Here, by deleting the branch-site adenosine (BS-A) or mutating the branch-site sequence of an actin pre-mRNA, we stall the assembly of spliceosomes in extracts from the yeast Saccharomyces cerevisiae directly before the A complex is formed. We then determine the three-dimensional structure of this newly identified assembly intermediate by cryo-electron microscopy. Our structure indicates that the U2–BS helix has formed in this pre-A complex, but is not yet clamped by the HEAT domain of the Hsh155 protein (Hsh155HEAT), which exhibits an open conformation. Thus, Prp5 proofreads the branch site indirectly, hindering spliceosome assembly if branch-site mutations prevent the remodelling of Hsh155HEAT.

To isolate a spliceosome assembly intermediate formed directly before the A complex that still contains Prp5, we carried out splicing in S. cerevisiae cell extracts with an actin (Act) pre-mRNA in which the BS-A is deleted. Spliceosomal complexes formed on ΔBS-A Act pre-mRNA lack the U4/U6.U5 tri-snRNP, but contain stoichiometric amounts of U1 and U2 snRNPs. The proteins Prp5, Msl5 and Mud2 are also abundant, whereas Cus2 is absent, indicating that these complexes stall after Prp5 hydrolyses ATP, but before the tri-snRNP has docked. We next carried out single-particle cryo-electron microscopy (cryo-EM) and determined the structure of the ΔBS-A complex at an average resolution of 5.9 Å (ranging from roughly 4.5 Å for U1 to approximately 15 Å for U2). By fitting known X-ray structures of spliceosome components into the EM density map, together with protein crosslinking coupled with mass spectrometry (CXMS), we generated a three-dimensional (3D) model of the ΔBS-A complex. This complex consists of two major elongated domains—comprising the U1 and bipartite U2 snRNPs—that are connected by two main bridges. In the pre-A complex, U1 and U2 are connected by a second bridge comprising intron nucleotides upstream of the branch site. Thus, formation of the U2–BS helix alone does not appear to trigger closure of Hsh155HEAT. As the U2–BS helix has formed, but Hsh155HEAT still exhibits an open conformation and Prp5 is stably bound (see below), we conclude that ΔBS-A complexes are stalled at a pre-A-complex stage, after Prp5-mediated formation of the U2–BS helix, but during/before it carries out its proofreading function. Comparison of our pre-A complex with the previously published yeast A complex15 reveals that the transition from the pre-A to the A complex involves large-scale remodelling that requires displacement of Prp5. The repositioning of U1 and the U2 3′-region is essential to generate the binding platform needed to dock the U4/U6.U5 tri-snRNP during formation of the pre-B complex.

> MSALYFQNLPSRPANKENYTRLLLKHINPNNKYAINPSLPLPHNKLQISSQPLMLLDDQMGLLEVSISRSSKMTNQAFLTFVTQEEADRFLEKYTTTALKVQGRKVRMGKARTNSLLGLSIEMQKKKGNDETYNLDIKKVLKARKLKRKLRSDDICAKKFRLKRQIRRLKHKLRSRKVEEAEIDRIVKEFETRRLENMKSQQENLKQSQKPLKRAKVSNTMENPPNKVLLIQNLPSGTTEQLLSQILGNEALVEIRLVSVRNLAFVEYETVADATKIKNQLGSTYKLQNNDVTIGFAK;> MNYNLSKYPDDVSRLFKPRPPLSYKRPTDYPYAKRQTNPNITGVANLLSTSLKHYMEEFPEGSPNNHLQRYEDIKLSKIKNAQLLDRRLQNWNPNVDPHIKDTDPYRTIFIGRLPYDLDEIELQKYFVKFGEIEKIRIVKDKITQKSKGYAFIVFKDPISSKMAFKEIGVHRGIQIKDRICIVDIERGRTVKYFKPRRLGGGLGGRGYSNRDSRLPGRFASASTSNPAERNYAPRLPRRETSSSAYSADRYGSSTLDARYRGNRPLLSAATPTAAVTSVYKSRNSRTRESQPAPKEAPDY;> MTRYYCEYCHSYLTHDTLSVRKSHLVGKNHLRITADYYRNKARDIINKHNHKRRHIGKRGRKERENSSQNETLKVTCLSNKEKRHIMHVKKMNQKELAQTSIDTLKLLYDGSPGYSKVFVDANRFDIGDLVKASKLPQRANEKSAHHSFKQTSRSRDETCESNPFPRLNNPKKLEPPKILSQWSNTIPKTSIFYSVDILQTTIKESKKRMHSDGIRKPSSANGYKRRRYGN;> MPDETNFTIEDIEPRPDALRGLDTQFLQDNTALVQAYRGLDWSDISSLTQMVDVIEQTVVKYGNPNDSIKLALETILWQILRKYPLLFGFWKRFATIEYQLFGLKKSIAVLATSVKWFPTSLELWCDYLNVLCVNNPNETDFIRNNFEIAKDLIGKQFLSHPFWDKFIEFEVGQKNWHNVQRIYEYIIEVPLHQYARFFTSYKKFLNEKNLKTTRNIDIVLRKTQTTVNEIWQFESKIKQPFFNLGQVLNDDLENWSRYLKFVTDPSKSLDKEFVMSVFDRCLIPCLYHENTWMMYIKWLTKKNISDEVVVDIYQKANTFLPLDFKTLRYDFLRFLKRKYRSNNTLFNNIFNETVSRYLKIWPNDILLMTEYLCMLKRHSFKNSLDQSPKEILEKQTSFTKILETSITNYINNQIDAKVHLQTLINDKNLSIVVVELIKTTWLVLKNNMQTRKYFNLYQKNILIKNSVPFWLTYYKFEKSNVNFTKLNKFIRELGVEIYLPTTVMNDILTDYKTFYLTHSNIVTYESSIIDSNTFDPILYPELKMSNPKYDPVLNTTANVDWHKKTEWKEAGHIGITTERPQISNSIIECNSGTLIQKPISLPNFRNLEKINQVKINDLYTEEFLKEGK;> MDKYTALIHDENFSTLTLNVSRYPKSLAYWEKLLNYIVKASAPICKSTEPQLLKLIRCTYSSMLNEFPYLENYYIDFALLEYKLGNVSMSHKIFQRGLQAFNQRSLLLWTSYLKFCNNVISHQKQLFKKYETAEEYVGLHFFSGEFWDLYLEQISSRCTSSKKYWNVLRKILEIPLHSFSKFYALWLQRIDDIMDLKQLSQLTSKDELLKKLKIDINYSGRKGPYLQDAKKKLKKITKEMYMVVQYQVLEIYSIFESKIYINYYTSPETLVSSDEIETWIKYLDYTITLQTDSLTHLNFQRALLPLAHYDLVWIKYSKWLINSKNDLLGAKNVLLMGLKFSLKKTEIIKLLYSVICKLNEYVLLRNLLEKIESSYSDNVENVDDFEIFWDYLQFKTFCQNSLYSSRYSDSQSNGLLNKELFDKVWKRLSCKEKKSGQEILLNNLVQFYSKDTVEFVEKNIFQKIIEFGWEYYLQNGMFWNCYCRLIYFDTSRSYLDKRQYIVRKIWPQIDKKFAQSVLPSLTEFCESYFPEEMDTLEEMFTEEP;> MSYKQTTYYPSRGNLVRNDSSPYTNTISSETNNSSTSVLSLQGASNVSLGTTGNQLYMGDLDPTWDKNTVRQIWASLGEANINVRMMWNNTLNNGSRSSMGPKNNQGYCFVDFPSSTHAANALLKNGMLIPNFPNKKLKLNWATSSYSNSNNSLNNVKSGNNCSIFVGDLAPNVTESQLFELFINRYASTSHAKIVHDQVTGMSKGYGFVKFTNSDEQQLALSEMQGVFLNGRAIKVGPTSGQQQHVSGNNDYNRSSSSLNNENVDSRFLSKGQSFLSNGNNNMGFKRNHMSQFIYPVQQQPSLNHFTDPNNTTVFIGGLSSLVTEDELRAYFQPFGTIVYVKIPVGKCCGFVQYVDRLSAEAAIAGMQGFPIANSRVRLSWGRSAKQTALLQQAMLSNSLQVQQQQPGLQQPNYGYIPSSTCEAPVLPDNNVSSTMLPGCQILNYSNPYANANGLGSNNFSFYSNNNATNTQATSLLADTSSMDLSGTGGQQVIMQGSEAVVNSTNAMLNRLEQGSNGFMFA;> MRPRRRGLAYHHTKPKGQLSQGHYPTTSNDGQRRKVGNSEAFQSFDIWKNLDRIRSTKKNAGQFIKGSLLILPMRTEDKQQFDECMDELHKYISKDILRCYPQKEQKDEGMLFYIVLKDFNILDSCFVLSVLLAFQKRLWMAPSEKSYFRVPKNINLTGSFYLPKNIETGRGHIITSYRREQPSSSIVEVGFNVVPDFQQFQVKACHVSKFMNELSNFFSQVEFGKCEANVINYFKREYNRTYSQISLALYELPLIGDGLFDIKSYISKTRPIIETSKAQMIKHISEMKAYNEISGLQGDQFPRQQRPLSNSPSSNSISSSQTIEAGATSYQTQPQRHAVNKPSNVLNSSNRHSGPKTFEDGRYSEGNKPGFMTQDEIKQHCIGTIKASMDAVKKKSSYQILKTYVRCPRQNYIDIVYQNLNDLRSKTNCNIVVLNLNNLHESQMWLESLNTTNYTIFAQAPHPSTIRVISIGGVGEYIVKALELILNILEH;> MSTMSTPAAEQRKLVEQLMGRDFSFRHNRYSHQKRDLGLHDPKICKSYLVGECPYDLFQGTKQSLGKCPQMHLTKHKIQYEREVKQGKTFPEFEREYLAILSRFVNECNGQISVALQNLKHTAEERMKIQQVTEELDVLDVRIGLMGQEIDSLIRADEVSMGMLQSVKLQELISKRKEVAKRVRNITENVGQSAQQKLQVCEVCGAYLSRLDTDRRLADHFLGKIHLGYVKMREDYDRLMKNNRTTNASKTATTLPGRRFV;> MRDIVFVSPQLYLSSQEGWKSDSAKSGFIPILKNDLQRFQDSLKHIVDARNSLSETLLNSNDDGSIHNSDQNTGLNKDKEASIADNNSANKCATSSSRYQELKQFLPISLDQQIHTVSLQGVSSSFSRGQIESLLDHCLNLALTETQSNSALKVEAWSSFSSFLDTQDIFIRFSKVDEDEAFVNTLNYCKALFAFIRKLHEDFKIELHLDLNTKEYVEDRTGTIPSVKPEKASEFYSVFKNIEDQTDERNSKKEQLDDSSTQYKVDTNTLSDLPSDALDQLCKDIIEFRTKVVSIEKEKKMKSTYEESRRQRHQMQKVFDQIRKNHSGAKGSANTEEEDTNMEDEDEEDDTEDDLALEKRKEERDLEESNRRYEDMLHQLHSNTEPKIKSIRADIMSAENYEEHLEKNRSLYLKELLHLANDVHYDHHRSFKEQEERRDEEDRAKNGNAKELAPIQLSDGKAISAGKAAAITLPEGTVKSENYNADKNVSESSEHVKIKFDFKKAIDHSVESSSEDEGYRESELPPTKPSERSAAEDRLPFTADELNIRLTNLKESRYVDELVREFLGVYEDELVEYILENIRVNQSKQALLNELRETFDEDGETIADRLWSRKEFRLGT;> MSIWKEAKDASGRIYYYNTLTKKSTWEKPKELISQEELLLRENGWKAAKTADGKVYYYNPTTRETSWTIPAFEKKVEPIAEQKHDTVSHAQVNGNRIALTAGEKQEPGRTINEEESQYANNSKLLNVRRRTKEEAEKEFITMLKENQVDSTWSFSRIISELGTRDPRYWMVDDDPLWKKEMFEKYLSNRSADQLLKEHNETSKFKEAFQKMLQNNSHIKYYTRWPTAKRLIADEPIYKHSVVNEKTKRQTFQDYIDTLIDTQKESKKKLKTQALKELREYLNGIITTSSSETFITWQQLLNHYVFDKSKRYMANRHFKVLTHEDVLNEYLKIVNTIENDLQNKLNELRLRNYTRDRIARDNFKSLLREVPIKIKANTRWSDIYPHIKSDPRFLHMLGRNGSSCLDLFLDFVDEQRMYIFAQRSIAQQTLIDQNFEWNDADSDEITKQNIEKVLENDRKFDKVDKEDISLIVDGLIKQRNEKIQQKLQNERRILEQKKHYFWLLLQRTYTKTGKPKPSTWDLASKELGESLEYKALGDEDNIRRQIFEDFKPESSAPTAESATANLTLTASKKRHLTPAVELDY;> MSHPIQFVNANNSDKSHQLGGQYSIPQDLRENLQKEAARIGENEKDVLQEKMETRTVQNREDSYHKRRFDMKFEPDSDTQTVTSSENTQDAVVPRKRKSRWDVKGYEPPDESSTAVKENSDSALVNVEGIHDLMFFKPSDHKYFADVISKKPIDELNKDEKKERTLSMLLLKIKNGNTASRRTSMRILTDKAVTFGPEMIFNRLLPILLDRSLEDQERHLMIKTIDRVLYQLGDLTKPYVHKILVVAAPLLIDEDPMVRSTGQEIITNLSTVAGLKTILTVMRPDIENEDEYVRNVTSRAAAVVAKALGVNQLLPFINAACHSRKSWKARHTGIKIVQQIGILLGIGVLNHLTGLMSCIKDCLMDDHVPVRIVTAHTLSTLAENSYPYGIEVFNVVLEPLWKGIRSHRGKVLSSFLKAVGSMIPLMDPEYAGYYTTEAMRIIRREFDSPDDEMKKTILLVLQKCSAVESITPKFLREEIAPEFFQKFWVRRVALDRPLNKVVTYTTVTLAKKLGCSYTIDKLLTPLRDEAEPFRTMAVHAVTRTVNLLGTADLDERLETRLIDALLIAFQEQTNSDSIIFKGFGAVTVSLDIRMKPFLAPIVSTILNHLKHKTPLVRQHAADLCAILIPVIKNCHEFEMLNKLNIILYESLGEVYPEVLGSIINAMYCITSVMDLDKLQPPINQILPTLTPILRNKHRKVEVNTIKFVGLIGKLAPTYAPPKEWMRICFELLELLKSTNKEIRRSANATFGFIAEAIGPHDVLVALLNNLKVQERQLRVCTAVAIGIVAKVCGPYNVLPVIMNEYTTPETNVQNGVLKAMSFMFEYIGNMSKDYIYFITPLLEDALTDRDLVHRQTASNVITHLALNCSGTGHEDAFIHLMNLLIPNIFETSPHAIMRILEGLEALSQALGPGLFMNYIWAGLFHPAKNVRKAFWRVYNNMYVMYQDAMVPFYPVTPDNNEEYIEELDLVL;> MWGGGKMAVVSLSPHTAKMRKLFGQASTTMAYDGLKREAERRTRSDHNITMVAKDDELYLYHLTLKKQTNFVHSCIGHFVDLEAGSKREQSQLCVATETHLELYDTADGELKLIAKFQNLFATITSMKSLDLPHSGSRAKASNWPTFLALTSDSGNLSIVQIIMHAGALRLKTLVNQPLTRTTLRRVSPISYMEIDPNGRCIILSSVEQNKLCFLVDYAQKLRISSPLEIIRPHMVTLDMAVVDVNFNNPCFVTLEIDNAATQLSVHLIFYVLELGLNHIVKKADYLVNPSANFVLSLPDLSRYNITTSLSDNNYDADYDTLFNPFVVIGFENHILVKDMNGFFSLKVEIPKRSITNSRHKNVTIISGIVQKLKNDFFVLLQSNHGDLFKLTVSPDTNDRNRPLVQLSYFDTIQNSHQLHIFKNGYLFALSEMNNNFLFQFEKLGVEKNDFSNVLTSKDPNKSLVFEPSIKLQNLSILSQQLNLNPSIKSQIVSDSPLSIATKHFTNNKIITLTNAVNYSNLISTSLPPNATKLWLIPDPATTGDNNTLLFITFPKKTMILQIDNESMEELTPDEATRSAFKLSQDTTIHTCLMGSHSIIQVCTAELRHIVPTGKSRYSNKLTWVPPAGIRIVCATSSKTQLIISLSNYELVYFKIDVSSDSLIELTTHPELDTMPSKVAIVQDTQHADLLAIADNEGMIKIMSLKDQKEDFLTVISLQLVSEKISDMIMVRDSSIGQLNLHVGLENGVYMKFHIGDVDGSFTDIKRRFLGLKPVSLSYLREISVSLNNEEEEEEEEDDDDEKEEEEINSSGAKWMSCVVCHSSSTWVSYTWKNVWTIRQLKDQNMLSCSKFVNADVAINGVCSISSSGRLNIGRVSNFPTLDNWFHVHESSVNKQENGGGDESNEEEEDEMEEEMEMLQISTFRPRTILSFPNNPKSILFIDNHSGKKQCRISLQIDGECLKFGSSDHLYKILDDIDCVSAAIIDFTRQADHLIICAGDKRLLTYKILVNKDKLSFDIELLHQTEIISPIHAMLKFKNFLLTAMGSTIVLYGLGKKQLLRRSVTQTPVSITKIVSMHQWNYERLAVGDIHESVTLFIWDPAGNVFIPYVDDSVKRHVTVLKFLDEATVIGADRYGNAWTLRSPPECEKIMSNHDPSELSNGAIKYPLDVITLQQKLPNTYDCKFKFQLLNHFFVNDIITDFHILDSLSNSDRPGCIYMGLQGTVGCFIPLLSKGNVFMMGNIENIMAEADDTFYLDYESRKKNNNMRKEDDEEESGSVVLQGRHGIEDEIICEGSCSILGRDHQEYRSYYAPVRKVIDGDLCENFLRLSLNEQEFLAKNLKSVQVEDIIQTINEVRTNYM;> MARTKSRKRSGNNQNKNASVVNNKAEIAAMIDARRLEQKKKGGVTNSKGKTNKVVDAKLEKEFKDVLQRFQVQENDTPKEITKDEKNNHVVIVEKNPVMNRKHTAEDELEDTPSDGIEEHLSARKRRKTEKPSLSQLKSQVPYPQIIEWYDCDARYPGLLASIKCTKNVIPVPSHWQSKKEYLSGRSLLGKRPFELPDIIKKTNIEQMRSTLPQSGLDGQDEKSLKEASRARVQPKMGALDLDYKKLHDVFFKIGANWKPDHLLCFGDVYYENRNLFEETNWKRMVDHKRPGRISQELRAIMNLPEGQLPPWCMKMKDIGLPTGYPDLKIAGLNWDITNLKGDVYGKIIPNHHSRSKKQGRNYFGALISFETPEFENSKEDTQANAENGRQDDKIDDEVEHKLDHFQEDISEVTSAEEKLERNEEESEKQLYTVLK;> MNYSADSGNTVYVGNIDPRITKEQLYELFIQINPVLRIKYPKDKVLQAYQGYAFIEFYNQGDAQYAIKIMNNTVRLYDRLIKVRQVTNSTGTTNLPSNISKDMILPIAKLFIKNLADSIDSDQLVKIFNKFGKLIREPEIFYLSNGKLKCAYVYFEDFEKADLAIKSLNNQLVANNRITVDYAFKENGKGNAKYGDDVDRLLNKEALKHNMLK;> MSRHQFDLIMCLKQPGVQTGLLCEKCDGKCPICDSYVRPKRKVRVCENCSFGKQAKNCIICNLNVGVNDAFYCWECCRLGKDKDGCPRILNLGSNRLDRHFEKKKKV;> MNLLETRRSLLEEMEIIENAIAERIQRNPELYYHYIQESSKVFPDTKLPRSSLIAENKIYKFKKVKRKRKQIILQQHEINIFLRDYQEKQQTFNKINRPEETQEDDKDLPNFERKLQQLEKELKNEDENFELDINSKKDKYALFSSSSDPSRRTNILSDRARDLDLNEIFTRDEQYGEYMELEQFHSLWLNVIKRGDCSLLQFLDILELFLDDEKYLLTPPMDRKNDRYMAFLLKLSKYVETFFFKSYALLDAAAVENLIKSDFEHSYCRGSLRSEAKGIYCPFCSRWFKTSSVFESHLVGKIHKKNESKRRNFVYSEYKLHRYLKYLNDEFSRTRSFVERKLAFTANERMAEMDILTQKYEAPAYDSTEKEGAEQVDGEQRDGQLQEEHLSGKSFDMPLGPDGLPMPYWLYKLHGLDREYRCEICSNKVYNGRRTFERHFNEERHIYHLRCLGIEPSSVFKGITKIKEAQELWKNMQGQSQLTSIAAVPPKPNPSQLKVPTELELEEEDEEGNVMSKKVYDELKKQGLV;> MNYLEGVGSKKGGGGIASESQFNLQRRKEVESLLSKGENVPYTFQDEKDDQVRSNPYIYKNHSGKLVCKLCNTMHMSWSSVERHLGGKKHGLNVLRRGISIEKSSLGREGQTTHDFRQQQKXXXXXXXXXXXXXXXXIIEAKQSLKNNGTIPVCKIATVKNPKNGSVGLAIQVNYSSEVKENSVDSDDKAKVPPLIRIVSGLELSDTKQKGKKFLVIAYEPFENIAIELPPNEILFSENNDMDNNNDGVDELNKKCTFWDAISKLYYVQFFFKQAEQEQADV;> MEPEDTQLKEDIKTTVNYIKQHGVEFENKLLEDERFSFIKKDDPLHEYYTKLMNEPTDTVSGEDNDRKSEREIARPPDFLFSQYDTGISRRDMEVIKLTARYYAKDKSIVEQMISKDGEARLNFMNSSHPLHKTFTDFVAQYKRVYSFTGQEIKKSKRTILDNCFERTQYWEFEKDKDREHDKLVELCKIQFAAIPWDKFTQVAKFSIPEDTEIFEGSLDLEQMRLRRVQTGIKLFDSIKPTNEEEKIVSDQGKQKGGDSKGKKRKIRAVGETRLKKSKK;> MKFTPSIVIDAPQYYVDHFNGKYNVDKCVILRDLQLETDSESMPSSLKHLTKPTHILDLTNNDLIMIPDLSRRDDIHTLLLGRNNIVEVDGRLLPMNVQNLTLSNNSIRRFEDLQRLRRAPRTLKNLTLIGNQVCHLANYREHVLRLVPHLETLDFQNVTAEERKSAMSFPRQADGDTLGPVNTAIRDNGSRDKTMEIMNLVVSKMTVERRNELKKQLAEATSLEEIARLEKLLSGGV;> MVEPARKKQRIDRDTHHTVAEPVTEAKNTLYVSQLNEKINMQRLRVNLFLLFATFGEVLKVSMNFKKQRGQAFITMRTIDQASLAQISLNGERFFGKPLKVEFSKSETKTL;> MAEKQRQLKLQKIYKQKYIGLGDESTTREQWQRNVRNDTLNTLQGHSASLEYVSLSRGDLSIRDTRIHLLKSMSPGYKAYLREER;>MSKIQVAHSSRLANLIDYKLRVLTQDGRVYIGQLMAFDKHMNLVLNECIEERVPKTQLDKLRPRKDSKDGTTLNIKVEKRVLGLTILRGEQILSTVVEDKPLLSKKERLVRDKKEKKQAQKQTKLRKEKEKKPGKIAKPNTANAKHTSSNSREIAQPSSSRYNGGNDNIGANRSRFNNEAPPQTRKFQPPPGFKRK[2x];>MTMNGIPVKLLNEAQGHIVSLELTTGATYRGKLVESEDSMNVQLRDVIATEPQGAVTHMDQIFVRGSQIKFIVVPDLLKNAPLFKKNSSRPMPPIRGPKRR[2x];>[2x]MSNKVKTKAMVPPINCIFNFLQQQTPVTIWLFEQIGIRIKGKIVGFDEFMNVVIDEAVEIPVNSADGKEDVEKGTPLGKILLKGDNITLITSAD;>[2x]MSESSDISAMQPVNPKPFLKGLVNHRVGVKLKFNSTEYRGTLVSTDNYFNLQLNEAEEFVAGVSHGTLGEIFIRCNNVLYIRELPN;>[2x]MVSTPELKKYMDKKILLNINGSRKVAGILRGYDIFLNVVLDDAMEINGEDPANNHQLGLQTVIRGNSIISLEALDAI;>[2x]MKLVNFLKKLRNEQVTIELKNGTTVWGTLQSVSPQMNAILTDVKLTLPQPRLNKLNSNGIAMASLYLTGGQQPTASDNIASLQYINIRGNTIRQIILPDSLNLDSLLVDQKQLNSLRRSGQIANDPSKKRRRDFGAPANKRPRRGL;>[2x]MSSQIIDRPKHELSRAELEELEEFEFKHGPMSLINDAMVTRTPVIISLRNNHKIIARVKAFDRHCNMVLENVKELWTEKKGKNVINRERFISKLFLRGDSVIVVLKTPVE;> METIDSKQNINRESLLEERRKKLAKWKQKKAQFDAQKEHQTSRNDIVTNSLEGKQTTEKFTERQERVKEELRKRKNEFRKSDEPVSVKPSKKKSKRSKVKKKISFDFSDDDDSEIGVSFRSKEHIQKAPEHDNEKDPLDEFMTSLKEEKMSNSKGMYDRGDILDVEDQLFELGGTDDEDVEDNTDNSNIAKIAKLKAKKRVKQIYYSPEELEPFQKNFYIESETVSSMSEMEVEELRLSLDNIKIKGTGCPKPVTKWSQLGLSTDTMVLITEKLHFGSLTPIQSQALPAIMSGRDVIGISKTGSGKTISYLLPLLRQVKAQRPLSKHETGPMGLILAPTRELALQIHEEVTKFTEADTSIRSVCCTGGSEMKKQITDLKRGTEIVVATPGRFIDILTLNDGKLLSTKRITFVVMDEADRLFDLGFEPQITQIMKTVRPDKQCVLFSATFPNKLRSFAVRVLHSPISITINSKGMVNENVKQKFRICHSEDEKFDNLVQLIHERSEFFDEVQSENDGQSSDVEEVDAKAIIFVSSQNICDFISKKLLNAGIVTCAIHAGKPYQERLMNLEKFKREKNSILLCTEVLSRGLNVPEVSLVIIYNAVKTFAQYVHTTGRTARGSRSGTAITLLLHDELSGAYILSKAMRDEEIKALDPLQAKELQEMSAKFESGMKKGKFRLSKGFGGKGLENIKSKREEAQNKDLELKKNDKRSDDLEKKISNPREGHDSVSESSALIPRLNYELFKESTDGSIIFYAKVYINDLPQIVRWEATKNTTLLFIKHETGCSITNKGKFYPEGKEPKNENDEPKLYLLIEGQDEKDIQLSIELLEQKVKEGVVKAASLSLKSTKY> MTKILVVLLSFSFLVSFFGINALLPTKAYAANSHDENFSPETLKFLRTNTGLDGEQWDNIMKLINKPEQDSLDWTKYYGYCEDIGDDRGYTIGIFGATTGGSNDKHPDGPTLFKEFDAASGAAN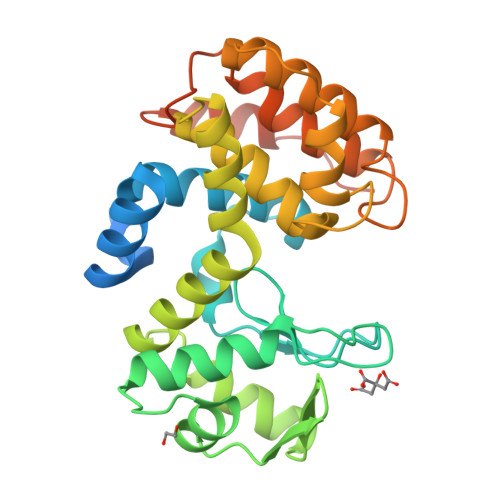PSVEGGLARIGVNGSMKGSILKIKDSEKVFCGKIKKLQNNDTWREAIWQTFYKVYIKYSVQQARQRGFNSALTIGSFVDTALNQGATGDSGTLQGILSRSGKSTDEKTFMKKFYAERTLVVDTNDYNQPPNGKNRVKQWSQLWDMGKADLKNADDAIVKVTSWKMKKSSVDKLAAALEHHHHHH>MSLETAYKPFLASSALVPTTPTAFQNELKTFRDSLISSCKKKNILITDTSSWLGFQVYSTQAPSVQAASTLGFELKAINSLVNKLAECGLSKFIKVYRPQLPIETPANNPEESDEADQAPWTPMPLEIAFQGDRESVLKAMNAITGMQDYLFTVNSIRIRNERMMPPPIANPAAAKPAAAQPATGAASLTPADEAAA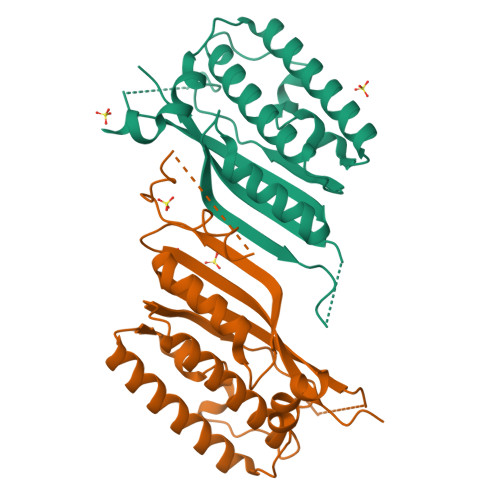PAAPAIQQVIKPYMGKEQVFVQVSLNLVHFNQPKAQEPSEDLEHHHHHH[2x]>[4x]TKHKERVMYYGKGDVFAYRTYLKPLTGVRTIPESPFSGRDHILFGVNVKISVGGTKLLTSFTKGDNSLVVATDSMKNFIQKHLASYTGTTIEGFLEYVATSFLKKYSHIEKISLIGEEIPFETTFAVKNGNRAASELVFKKSRNEYATAYLNMVRNEDNTLNITEQQSG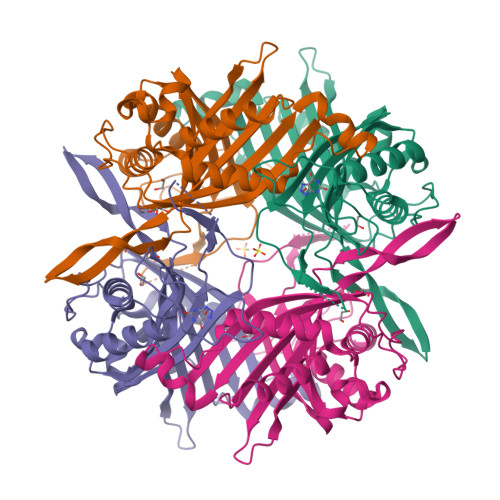LAGLQLIKVSGNSFVGFIRDEYTTLPEDSNRPLFVYLNIKWKYKNTEDSFGTNPENYVAAEQIRDIATSVFHETETLSIQHLIYLIGRRILERFPQLQEVYFESQNHTWDKIVEEIGESEGKVYTEPRPPYGFQCFTVTQEDLPHENILMFSDEPDHKGALK> AAPTAYTPLDVAQAYQFPEGLDGQGQCIAIIELGGGYDEASLAQYFASLGVPAPQVVSVSVDGASNQPTGDPSGPDGEVELDIEVAGALAPGAKFAVYFAPNTDAGFLDAITTAIHDPTLKPSVVSISWGGPEDSWTSAAIAAMNRAFLDAAALGVTVLAAAGDSGSTDGEQDGLYHVDFPAASPYVLACGGTRLVASGGRIAQETVWNDGPDGGATGGGVSRIFPLPAWQEHANVPPSANPGASSGRGVPDLAGNADPATGYEVVIDGEATVIGGTSAV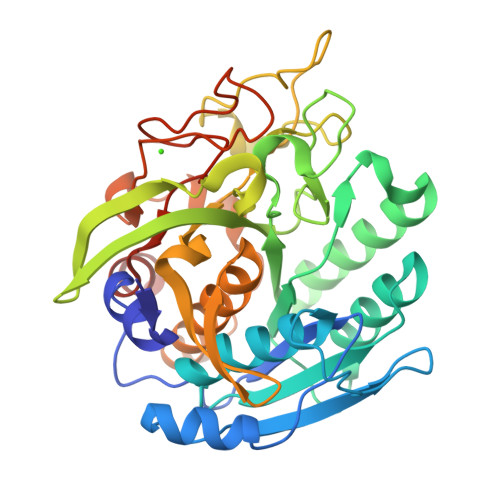APLFAALVARINQKLGKAVGYLNPTLYQLPADVFHDITEGNNDIANRAQIYQAGPGWDPCTGLGSPIGVRLLQALLPSASQPQP>MTNILIVEDDPMVQFIHRNYLEKIGTFDTIYSSETIADAKKLLASRSIQLVLLDIRLKDGNGIDFLTDLRRTKQTVDVILITAANEVNIVNDALHLGVIDYLIKPFTLERFEKSIQRY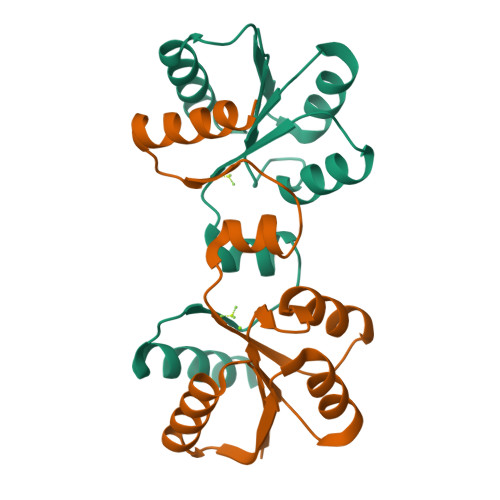RTKH[2x]>ADKELKFLVVDDFSTMRRIVRNLLKELGFNNVEEAEDGVDALNKLQAGGYGFVISDWNMPNMDGLELLKTIRADGAMSALPVLMVTAEAKKENIIAA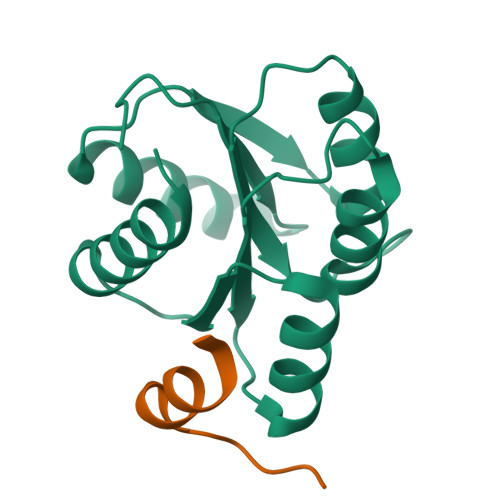AQAGASGYVVKPFTAATLEEKLNKIFEKLGM[2x];>MGDSILSQAEIDALLN[2x]>SLTDSVYERLLSERIIFLGSEVNDEIANRLCAQILLLAAEDASKDISLYINSPGGSISAGMAIYDTMVLAPCDIATYAMGMAASMGEFLLAAGTKGKRYALPHARILMHQPLGGVTGSAADIAIQAEQFAVIKKEMFRLNAEFTGQPIERIEADSDRDRWFTAAEALEYGFVDHIITR[7x];>[7x]NPYNKLFEERIIFLGVQVDDASANDIMAQLLVLESLDPDRDITMYINSPGGGFTSLMAIYDTMQYVRADIQTVCLGQAASAAAVLLAAGTPGKRMALPNARVLIHQPSLSGVIQGQFSDLEIQAA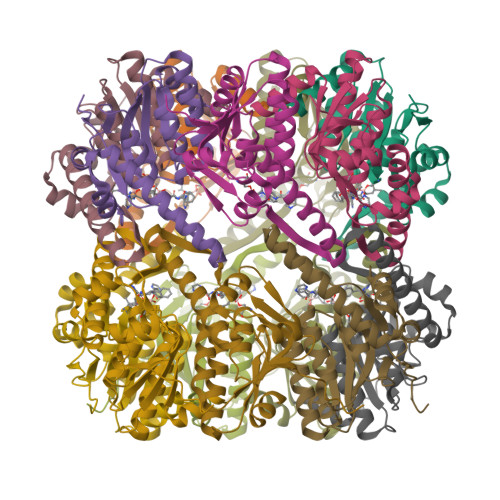EIERMRTLMETTLARHTGKDAGVIRKDTDRDKILTAEEAKDYGIIDTVLEYRKLS propan-2-yl (2~{S})-2-[[2,6-bis(chloranyl)phenyl]-(furan-2-ylcarbonyl)amino]propanoate | C17 H17 Cl2 N O4 | 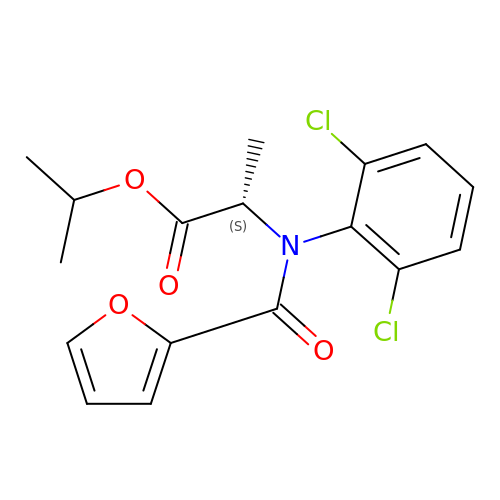QVXCXYZAVANRBK-NSHDSACASA-N ATP synthases use a transmembrane electrochemical proton motive force (pmf) to generate adenosine triphosphate (ATP) from adenosine diphosphate (ADP) and inorganic phosphate (Pi). ATP synthases are macromolecular machines consisting of an ATP-hydrolysis-driven F1 motor and a proton-translocation-driven FO motor. The F1 and FO motors oppose each other’s action on a shared rotor subcomplex and are held stationary relative to each other by a peripheral stalk. In Saccharomyces cerevisiae, the FO region contains subunits a, e, f, g, i/j, k, 8, part of subunit b, and the c10-ring of the rotor, while the F1 region includes a trimer of catalytic subunit αβ pairs and subunits γ, δ, and ε from the rotor.

We purified S. cerevisiae ATP synthase with the detergent n-Dodecyl-β-D-Maltopyranoside (DDM), which results in a monomeric preparation of the enzyme, and determined its structure by cryoEM. Three-dimensional (3D) classification allowed particle images to be separated into six rotor positions, corresponding to the catalytic and binding dwells for each of the three main rotational states. Further classification of the State 1catalytic conformation resulted in classes distinguished by variability in the position of the peripheral stalk and a slight rotation of the rotor relative to subunit a. These classes were designated as State 1catalytic(a) (light blue) to State 1catalytic(d) (dark blue) in order of increasing straightening of the peripheral stalk (‘no ATP’ condition). As these structures were determined in the absence of free ATP, they likely represent energetically similar conformations that can be reached by thermal fluctuation of the enzyme structure.

>[10x]MQLVLAAKYIGAGISTIGLLGAGIGIAIVFAALINGVSRNPSIKDTVFPMAILGFALSEATGLFCLMVSFLLLFGV;>ASTKAQPTEVSSILEERIKGVSDEANLNETGRVLAVGDGIARVFGLNNIQAEELVEFSSGVKGMALNLEPGQVGIVLFGSDRLVKEGELVKRTGNIVDVPVGPGLLGRVVDALGNPIDGKGPIDAAGRSRAQVKAPGILPRRSVHEPVQTGLKAVDALVPIGRGQRELIIGDRQTGKTAVALDTILNQKRWNNGSDESKKLYCVYVAVGQKRSTVAQLVQTLEQHDAMKYSIIVAATASEAAPLQYLAPFTAASIGEWFRDNGKHALIVYDDLSKQAVAYRQLSLLLRRPPGREAYPGDVFYLHSRLLERAAKLSEKEGSGSLTALPVIETQGGDVSAYIPTNVISITDGQIFLEAELFYKGIRPAINVGLSVSRVGSAAQVKALKQVAGSLKLFLAQYREVAAFAQFGSDLDASTKQTLVRGERLTQLLKQNQYSPLATEEQVPLIYAGVNGHLDGIELSRIGEFESSFLSYLKSNHNELLTEIREKGELSKELLASLKSATESFVATF[3x];>ASAAQSTPITGKVTAVIGAIVDVHFEQSELPAILNALEIKTPQGKLVLEVAQHLGENTVRTIAMDGTEGLVRGEKVLDTGGPISVPVGRETLGRIINVIGEPIDERGPIKSKLRKPIHADPPSFAEQSTSAEILETGIKVVDLLAPYARGGKIGLFGGAGVGKTVFIQELINNIAKAHGGFSVFTGVGERTREGNDLYREMKETGVINLEGESKVALVFGQMNEPPGARARVALTGLTIAEYFRDEEGQDVLLFIDNIFRFTQAGSEVSALLGRIPSAVGYQPTLATDMGLLQERITTTKKGSVTSVQAVYVPADDLTDPAPATTFAHLDATTVLSRGISELGIYPAVDPLDSKSRLLDAAVVGQEHYDVASKVQETLQTYKSLQDIIAILGMDELSEQDKLTVERARKIQRFLSQPFAVAEVFTGIPGKLVRLKDTVASFKAVLEGKYDNIPEHAFYMVGGIEDVVAKAEKLAAEAN[3x];> ATLKEVEMRLKSIKNIEKITKTMKIVASTRLSKAEKAKISAKKMDEAEQLFYKNAETKNLDVEATETGAPKELIVAITSDKGLCGSIHSQLAKAVRRHLNDQPNADIVTIGDKIKMQLLRTHPNNIKLSINGIGKDAPTFQESALIADKLLSVMKAGTYPKISIFYNDPVSSLSFEPSEKPIFNAKTIEQSPSFGKFEIDTDANVPRDLFEYTLANQMLTAMAQGYAAEISARRNAMDNASKNAGDMINRYSILYNRTRQAVITNELVDIITGASSLG;> AEAAAASSGLKLQFALPHETLYSGSEVTQVNLPAKSGRIGVLANHVPTVEQLLPGVVEVMEGSNSKKFFISGGFATVQPDSQLCVTAIEAFPLESFSQENIKNLLAEAKKNVSSSDAREAAEAAIQVEVLENLQSVLK;> SAWRKAGISYAAYLNVAAQAIRSSLKTELQTASVLNRSQTDAFYTQYKNGTAASEPTPITK;> ASKAAAPPPVRLFGVEGTYATALYQAAAKNSSIDAAFQSLQKVESTVKKNPKLGHLLLNPALSLKDRNSVIDAIVETHKNLDGYVVNLLKVLSENNRLGCFEKIASDFGVLNDAHNGLLKGTVTSAEPLDPKSFKRIEKALSASKLVGQGKSLKLENVVKPEIKGGLIVELGDKTVDLSISTKIQKLNKVLEDSI;> SPLDQFEIRTLFGLQSSFIDLSCLNLTTFSLYTIIVLLVITSLYTLTNNNNKIIGSRWLISQEAIYDTIMNMTKGQIGGKNWGLYFPMIFTLFMFIFIANLISMIPYSFALSAHLVFIISLSIVIWLGNTILGLYKHGWVFFSLFVPAGTPLPLVPLLVIIETLSYFARAISLGLRLGSNILAGHLLMVILAGLTFNFMLINLFTLVFGFVPLAMILAIMMLEFAIGIIQGYVWAILTASYLKDAVYLH;> MSSTPEKQTDPKAKANSIINAIPGNNILTKTGVLGTSAAAVIYAISNELYVINDESILLLTFLGFTGLVAKYLAPAYKDFADARMKKVSDVLNASRNKHVEAVKDRIDSVSQLQNVAETTKVLFDVSKETVELESEAFELKQKVELAHEAKAVLDSWVRYEASLRQLEQRQLAKSVISRVQSELGNPKFQEKVLQQSISEIEQLLSKLK;> SLAKSAANKLDWAKVISSLRITGSTATQLSSFKKRNDEARRQLLELQSQPTEVDFSHYRSVLKNTSVIDKIESYVKQYKPVKIDASKQLQVIESFEKHAMTNAKETESLVSKELKDLQSTLDNIQSARPFDELTVDDLTKIKPEIDAKVEEMVKKGKWDVPGYKDRFGNLNVM;> VSTLIPPKVVSSKNIGSAPNAKRIANVVHFYKSLPQGPAPAIKANTRLARYKAKYFDGDNASGKPLWHFALGIIAFGYSMEYYFHLRHHKGAEEH;> NVIQDLYLRELKDTKLAPSTLQDAEGNVKPWNPPQKPNLPELELQGPEALKAYTEQNVETAHVAKESEEGESEPIEEDWLVLDDAEETKESH;> MLKRFPTPILKVYWPFFVAGAAVYYGMSKAADLSSNTKEFINDPRNPRFAKGGKFVEVD;> MPQLVPFYFMNQLTYGFLLMITLLILFSQFFLPMILRLYVSRLFISKL However, intestinal bacterial GUSs cleave the attached glucuronic acid for use as a carbon source, allowing potentially toxic compounds to re-enter the enterohepatic circulation. However, microflora-encoding β-glucuronidases (GUSs) are notorious for reversing the glucuronidation to release SN-38 in the intestinal lumen and thus represent the major cause of undesirable effects. GUS contains a deep enzyme active site (the two catalytic glutamates lie ~12 Å below the protein surface). To understand the underlying structural basis, we prepared C6-propyl, -hexyl, and -nonyl UIFGs (2–4, respectively) and resolved the eight X-ray crystal structures of 1–4 bound to EcGUS or Bifidobacterium dentium GUS (BdGUS).

Isothermal titration calorimetry was used to measure the thermodynamics of the binding of 1 or 2 to EcGUS and BdGUS. At pH 8.0, the endocyclic amine of inhibitor 2 (pKa = 9.4) was mostly protonated, which afforded a stronger electrostatic interaction with catalytic residues than did 1 (pKa = 8.0). In addition to a small negative enthalpy change (about –2 to –4 kcal mol−1), binding was contributed mainly by entropy (+4.6 kcal mol−1 for BdGUS in Tris buffer; +7.1 and +5.0 kcal mol−1 for EcGUS in Tris and phosphate buffer, respectively). With the aforementioned structural information, the differences between the thermodynamic parameters for 1 and 2 support the idea that the lack of H-bonded water molecules for 2 diminished the coordinated H-bond network, which disfavored binding and thus the observed enthalpy penalty (ΔΔH1–2 = +8.5 kcal mol−1 for BdGUS in Tris buffer; +6.2 and +5.5 kcal mol−1 for EcGUS in Tris and phosphate buffer, respectively). Furthermore, the expulsion of water molecules also correlated with the entropy increase (i.e., –TΔΔS1–2 = −6.2 kcal mol−1 for BdGUS in Tris buffer; –5.6 and –4.6 kcal mol−1 for EcGUS in Tris and phosphate buffer, respectively). Therefore, introduction of an alkyl substituent to C6 of UIFG produced entropy-driven binding. Furthermore, EcGUS contains a narrower aglycone-binding site than LgGUS and BdGUS. The alkyl substituent of the inhibitors therefore facilitated an increase in hydrophobic contacts with nonpolar residues of loops 3 and 5 in EcGUS, e.g., such as Leu361, Phe365 in loop 3, and Val446, Met447, and Phe448 in loop 5.

> GSHMLRPVETPTREIKKLDGLWAFSLDRENCGIDQRWWESALQESRAIAVPGSFNDQFADADIRNYAGNVWYQREVFIPKGWAGQRIVLRFDAVTHYGKVWVNNQEVMEHQGGYTPFEADVTPYVIAGKSVRITVCVNNELNWQTIPPGMVITDENGKKKQSYFHDFFNYAGIHRSVMLYTTPNTWVDDITVVTHVAQDCNHASVDWQVVANGDVSVELRDADQQVVATGQGTSGTLQVVNPHLWQPGEGYLYELCVTAKSQTECDIYPLRVGIRSVAVKGEQFLINHKPFYFTGFGRHEDADLRGKGFDNVLMVHDHALMDWIGANSYRTSHYPYAEEMLDWADEHGIVVIDETAAVGFNLSLGIGFEAGNKPKELYSEEAVNGETQQAHLQAIKELIARDKNHPSVVMWSIANEPDTRPQGAREYFAPLAEATRKLDPTRPITCVNVMFCDAHTDTISDLFDVLCLNRYYGWYVQSGDLETAEKVLEKELLAWQEKLHQPIIITEYGVDTLAGLHSMYTDMWSEEYQCAWLDMYHRVFDRVSAVVGEQVWNFADFATSQGILRVGGNKKGIFTRDRKPKSAAFLLQKRWTGMNFGEKPQQGGKQ;> MLRPVETPTREIKKLDGLWAFSLDRENCGIDQRWWESALQESRAIAVPGSFNDQFADADIRNYAGNVWYQREVFIPKGWAGQRIVLRFDAVTHYGKVWVNNQEVMEHQGGYTPFEADVTPYVIAGKSVRITVCVNNELNWQTIPPGMVITDENGKKKQSYFHDFFNYAGIHRSVMLYTTPNTWVDDITVVTHVAQDCNHASVDWQVVANGDVSVELRDADQQVVATGQGTSGTLQVVNPHLWQPGEGYLYELCVTAKSQTECDIYPLRVGIRSVAVKGEQFLINHKPFYFTGFGRHEDADLRGKGFDNVLMVHDHALMDWIGANSYRTSHYPYAEEMLDWADEHGIVVIDETAAVGFNLSLGIGFEAGNKPKELYSEEAVNGETQQAHLQAIKELIARDKNHPSVVMWSIANEPDTRPQGAREYFAPLAEATRKLDPTRPITCVNVMFCDAHTDTISDLFDVLCLNRYYGWYVQSGDLETAEKVLEKELLAWQEKLHQPIIITEYGVDTLAGLHSMYTDMWSEEYQCAWLDMYHRVFDRVSAVVGEQVWNFADFATSQGILRVGGNKKGIFTRDRKPKSAAFLLQKRWTGMNFGEKPQQGGKQ>GQKKSIYVAYTGGTIGMQRSDNGYIPVSGHLQRQLALMPEFHDPEMPDFTIHEYAPLIDSSDMTPEDWQHIANDIQQNYDLYDGFVILHGTDTMAFTASALSFMLENLAKPVIITGSQIPLAELRSDGQTNLLNALYLAANHPVNEVSLFFNNQLFRGNRTTKAHADGFDAFASPNLSVLLEAGIHIRRQSSVVSPTSNGPLIVHRITPQPIGVVTIYPGISGAVVRNFLLQPVKALILRSY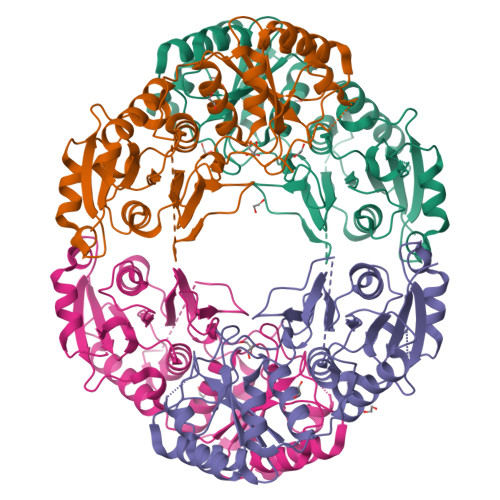GVGNAPQKAELLDELKNASDRGIVVVNLTQSISGSVNMGGYATGNALAQAGVISGFDMTVEAALTKLHYLLSQSLSPNEIRQLMQQNLRGELTDTQ[4x]> CCGG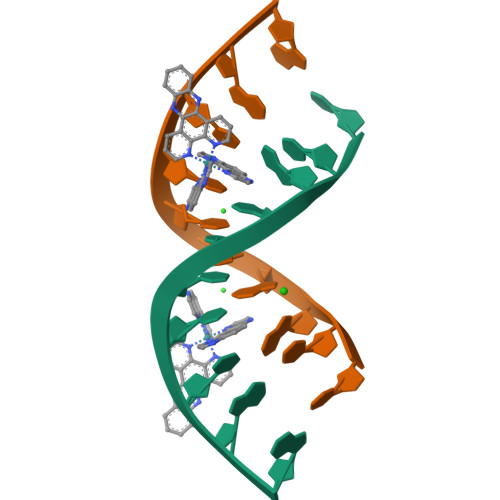ATCCGG> MLSQIAICIWVESTAILQDCQRALSADRYQLQVCESGEMLLEYAQTHRDQIDCLILVAANPSFRAVVQQLCFEGVVVPAIVVGDRDSEDPDEPAKEQLYHSAELHLGIHQLEQLPYQVDAALAEFLRLAPVETMADHIMLMGANHDPELSSQQRDLAQRLQERLGYLGVYYKRDPDRFLRNLPAYESQKLHQAMQTSYREIVLSYFSPNSNLNQSIDNFVNMAFFADVPVTKVVEIHMELMD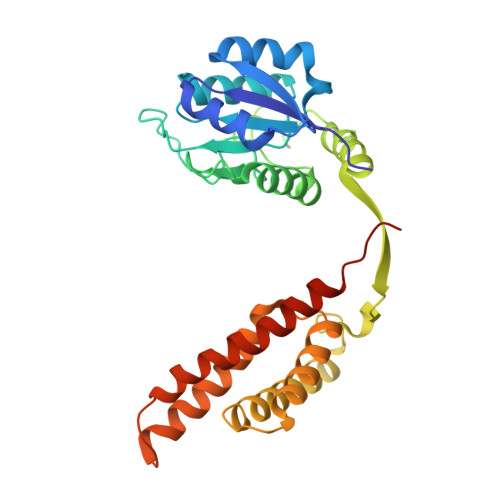EFAKKLRVEGRSEDILLDYRLTLIDVIAHLCEMYRRSIPRETHHHHHH5'-deoxy-5'-(dimethyl-lambda~4~-sulfanyl)adenosine | C12 H19 N5 O3 S | 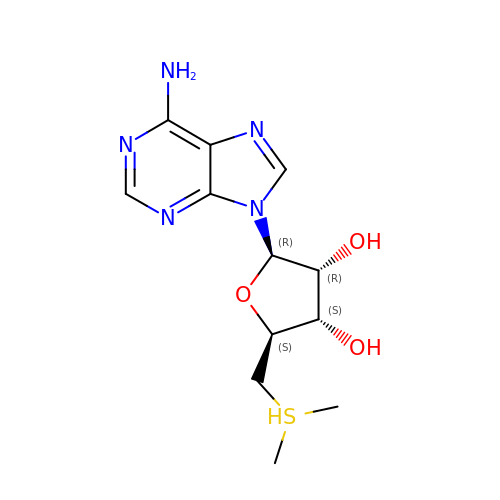QTJGMLRCRBTBIN-WOUKDFQISA-N> S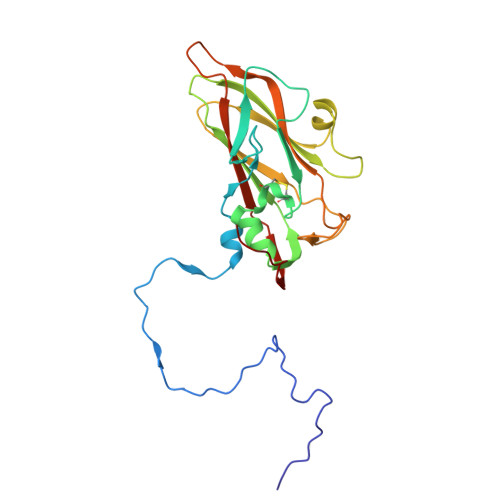PFPVTVREHAGTFFSTTPDTTVPVYGNTISTPFDYMCGEFTDLLSLCKIPTFLGNLDSNKKRIPYFSATNSTPATPLVTYQVTLSCSCMANSMLAAVARNFNQYRGSLNYLFVFTGSAMTKGKFLISYTPPGAGEPKTLDQAMQATYAIWDLGLNSSYNFTVPFISPTHYRQTSYNTPTITSVDGWLTVWQLTPLTYPLGVPNDSHILTLVSGGDDFTLRMPVTFTKYVPQ GlmM is a phosphoglucomutase enzyme catalyzing the conversion of glucosamine-6-phosphate to glucosamine-1-phosphate, which is subsequently used to produce the essential peptidoglycan precursor UDP-N-acetyl-glucosamine. CdaA (also referred to as DacA in some bacteria) is a membrane-bound cyclase with three predicted N-terminal transmembrane helices and a cytoplasmic catalytic DAC domain. c-di-AMP is formed from two molecules of ATP by enzymes containing a DAC domain. As part of the current study, we investigated how the activity the B. subtilis c-di-AMP cyclase CdaA is regulated by GlmM, a phosphoglucomutase enzyme required for the synthesis of an essential peptidoglycan precursor.

The B. subtilis GlmM protein displayed a four-domain architecture typical for phosphoglucosamine mutase proteins. Domains 1 to 3 are comprised of α-β mixed cores linked via a flexible loop to domain 4, which displays a three-stranded β sheet fold surrounded by two α-helices. While one GlmM molecule was present in the asymmetric unit, the typical “M-shaped” GlmM dimer arrangement was observed in the crystal cell packing. Interactions were formed between domains 1, leading to the formation of a large groove at the top of the dimer molecule, mostly formed by domain 2 and the active site of each monomer subunit facing the opposite direction. Two different structures were solved for the B. subtilis GlmM protein at 2.9 and 3.0 Å resolutions with a superposition r.m.s.d. score of 0.29. In the second structure, a phosphate molecule (PO4) was bound to Arg419, located within a loop region in domain 4 at a similar location as observed in the B. anthracis GlmM structure. The B. subtilis GlmM structure further highlighted the flexibility of the most C-terminal domain 4, which was found in the most open conformation seen in any GlmM protein structure up to date.

> MGKYFGTDGVRGVANSELTPELAFKVGRFGGYVLTKDKQRPKVLIGRDTRISGHMLEGALVAGLLSIGAEVMRLGVISTPGVSYLTKAMDAEAGVMISASHNPVQDNGIKFFGGDGFKLSDEQEAEIERLMDEPEDKLPRPVGADLGLVNDYFEGGQKYLQFLKQTADEDFTGIHVALDCANGATSSLATHLFADLDADVSTMGTSPNGLNINDGVGSTHPEALSAFVKEKNADLGLAFDGDGDRLIAVDEKGNIVDGDQIMYICSKHLKSEGRLKDDTVVSTVMSNLGFYKALEKEGIKSVQTAVGDRYVVEAMKKDGYNVGGEQSGHLIFLDYNTTGDGLLSAIMLMNTLKATGKPLSELAAEMQKFPQLLVNVRVTDKYKVEENEKVKAVISEVEKEMNGDGRILVRPSGTEPLVRVMAEAKTKELCDEYVNRIVEVVRSEMGLELVPRGSSGLEHHHHHH>[6x]YKKAGLQRTLVLIKPDAFERSLVAEIMGRIEKKNFKIVSMKFWSKAPRNLIEQHYKEHS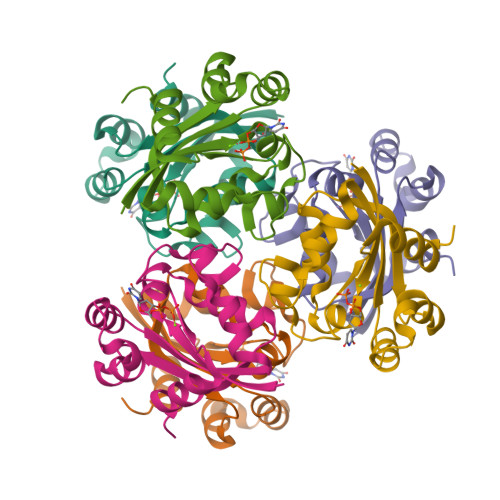EQSYFNDLCDFMVSGPIISIVYEGTDAISKIRRLQGNILTPGTIRGDLANDIRENLIHASDSEDSAVDEISIWFPETKMETDN> SKDPTTFPLGCSPDITTPKKGLSMELYSYDFRKKGSYPCWDAAYLDPNYPRTGYKSHRLLAKVDGVTGNINFYYHATKGCTPQLGHLPASYNY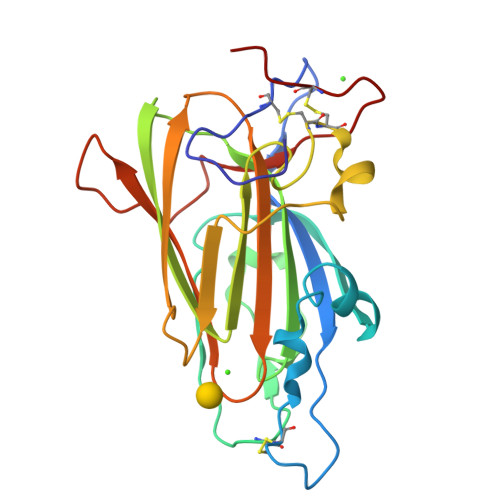PKPLTMTNFTMLLYGYFRPKVTGFHTFTISADDLLFVNFGAGNAFDCCRRDSSADHFGNYQAYAIWGSKTAKDELTVHLDAGVYYPIRLFYNNREYDGALSFTFKTESNENTVSDFSEYFFSLDDTEEGCPGLI> PSSVVRDVAIIGLSGRYPQAKNVDEFWNRLKEGKNCISEIPKDRWDWQSFFDEEKGKKESMYTKWGGFIDDMDKFDPLFFQISPKEAEEMDPQERLFLQEAYASIEDAGYTPTTLCESRKVGVFVGVMNGNYPTGATYWSIANRLSYLLNFQGPSVAVDTACSASLTAIHFALESLYSGTSECAIAGGVNLIVDPVHYMKLSALTMLSPSNQCKSFGDQADGFVDGEGVGAIVLKPLDKAIADGDHIYGVIKGSMMNAGGKTNGYTVPNPQAQAQLVADALQRANVHARTVSYLEAHGTGTELGDPIEVAGLTRAFEKDTQDKQFCALGSAKSNIGHCESA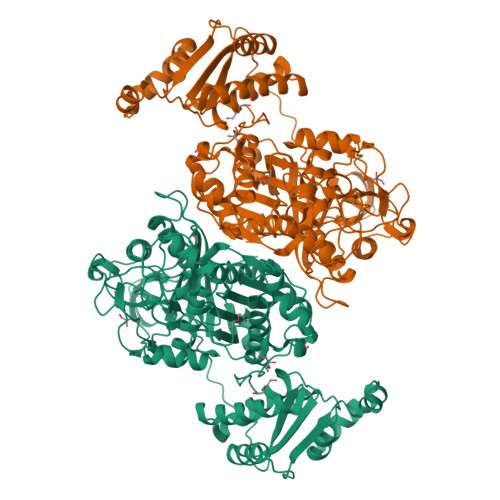AGIAGVTKILLQLKHAQLVPSLHSRTLNPNIDFTKTPFVVQQELAEWRRPIVEINGTTNEYPRIAGISSFGAGGSNAHVIIEEYIPEEQKQSSLKITPQNPAIFVLSAKNAERLYEIVQQLLAFIQEHSLSDEHLADMAYTLQVGRVAMEERIAVIAGTMKELQQKLTAYVKGQEHIADLYRGQVNRNQEMLDILTSDDELEETIARWMERGKYSKLLDLWVKGLSIDWNKLYQEEQPGRISLPTYPFAKESYWTHARSVSSSTGVGV> ATDKERFIASLMARMSNAEKIGQLRLVSVGADHPKEALMADIRAGKVGAIFNTVTRPDIRAMQDQVRHSRLKIPLFHAYDVAHGHRTIFPISLGLAASWDPEVVARSARISALEASADGLDMSFSPMVDITRDARWGRVSEGFGEDTYLTSLLSGVMVRAYQGSNLAAPDSIMAAVKHFA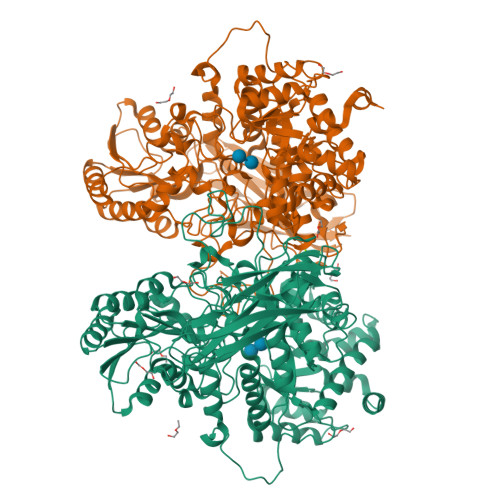LYGAAEGGRDYNTVDMSLPRMFQDYLPPYKAAVDAGAGAVMVSLNTINGVPATANRWLLTDLLRQQWGFKGLTISNHGAVKELIKHGLAGNERDATRLAIQAGVDMNMNDDLYSTWLPKLLAAGEIDQADIDRACRDVLAAKYDLGLFADPYRRLGKPDDPPFDTNAESRLHRQAAREVAREGLVLLKNRDGLLPLKKQGRIAVIGPLAKSQRDVIGSWSAAGVPRQAVTVYQGLANAVGERATLLYAKGANVSGDQAILDYLNSYNPEVEVDPRSAEAMLEEALRTARDADLVVAVVGESQGMAHEASSRTDLRIPASQRRLLKALKATGKPLVLVLMNGRPLSLGWEQENADAILETWFSGTEGGNAIADVLFGEHNPSGKLTMSFPRSVGQVPVYYNHLNTGRPMDHDNPGKYTSRYFDEANGPLYPFGYGLSYTEFSLSPLRLSSERLARGATLEARVTLSNSGKRAGATVVQLYLQDPVASLSRPVKELRGFRKVMLEPGESREIVFRLGEADLKFYDSQLRHTAEPGEFKVFVGLDSAQTESRSFTLL;> TDKERFIASLMARMSNAEKIGQLRLVSVGADHPKEALMADIRAGKVGAIFNTVTRPDIRAMQDQVRHSRLKIPLFHAYDVAHGHRTIFPISLGLAASWDPEVVARSARISALEASADGLDMSFSPMVDITRDARWGRVSEGFGEDTYLTSLLSGVMVRAYQGSNLAAPDSIMAAVKHFALYGAAEGGRDYNTVDMSLPRMFQDYLPPYKAAVDAGAGAVMVSLNTINGVPATANRWLLTDLLRQQWGFKGLTISNHGAVKELIKHGLAGNERDATRLAIQAGVDMNMNDDLYSTWLPKLLAAGEIDQADIDRACRDVLAAKYDLGLFADPYRRLGKPDDPPFDTNAESRLHRQAAREVAREGLVLLKNRDGLLPLKKQGRIAVIGPLAKSQRDVIGSWSAAGVPRQAVTVYQGLANAVGERATLLYAKGANVSGDQAILDYLNSYNPEVEVDPRSAEAMLEEALRTARDADLVVAVVGESQGMAHEASSRTDLRIPASQRRLLKALKATGKPLVLVLMNGRPLSLGWEQENADAILETWFSGTEGGNAIADVLFGEHNPSGKLTMSFPRSVGQVPVYYNHLNTGRPMDHDNPGKYTSRYFDEANGPLYPFGYGLSYTEFSLSPLRLSSERLARGATLEARVTLSNSGKRAGATVVQLYLQDPVASLSRPVKELRGFRKVMLEPGESREIVFRLGEADLKFYDSQLRHTAEPGEFKVFVGLDSAQTESRSFTLL>[2x]MKKIALIIGSMIAGGIISAAGFTWVAKAEPPAEKTSTAERKILFWYDPMYPNTRFDKPGKSPFMDMDLVPKYADEESSASGVRIDPTQTQNLGVKTATVTRGPLTFAQSFPANVSYNEYQYAIVQAR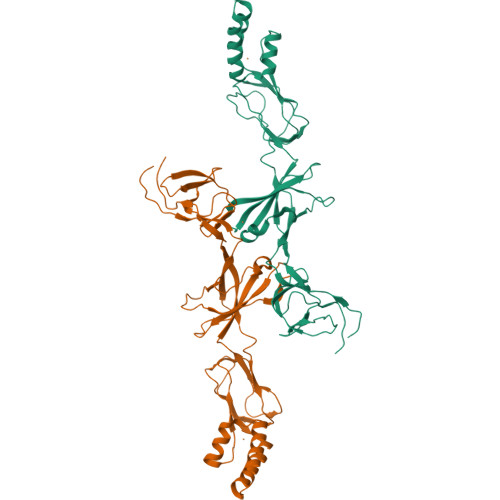AAGFIDKVYPLTVGDKVQKGTPLLDLTIPDWVEAQSEYLLLRETGGTATQTEGILERLRLAGMPEADIRRLIATQKIQTRFTLKAPIDGVITAFDLRAGMNIAKDNVVAKIQGMDPVWVTAAIPESIAWLVKDASQFTLTVPARPDKTLTIRKWTLLPGVDAATRTLQLRLEVDNADEALKPGMNAWLQLNTASEPMLLIPSQALIDTGSEQRVITVDADGRFVPKRVAVFQASQGVTALRSGLAEGEKVVSSGLFLIDSEANISGALERMRSESATHAHHHHHHH>GANPTTAETLDATRRVDDATVAIRCAINNLIVELIRGTGSYNRSSFESSSGLVWTSGPAGEGSYSITTPSQFVFLSSAWADPIELINLCTNALGNQFQTQQARTVVQRQF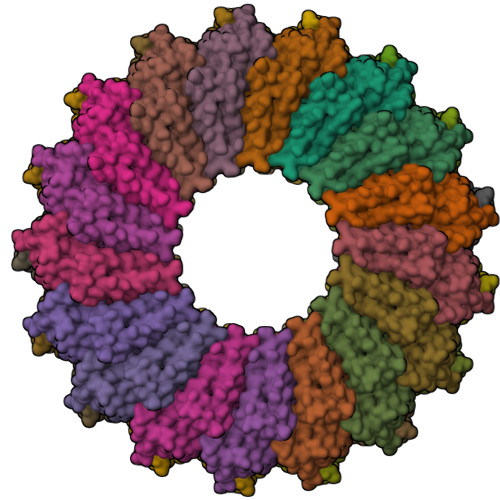SEVWKPSPQVTVRFPDSDFKVYRYNAVLDPLVTALLGAFDTRNRIIEVENQ[17x]>GPGSTEPFGLDRGLELDKVLHCYQMKELFLFVTWKGCSSIDAVPMKYIREAYPLQVIEFFQSGSGSGS[2x];>[2x]MENLAKIRMSQKLACWQQIL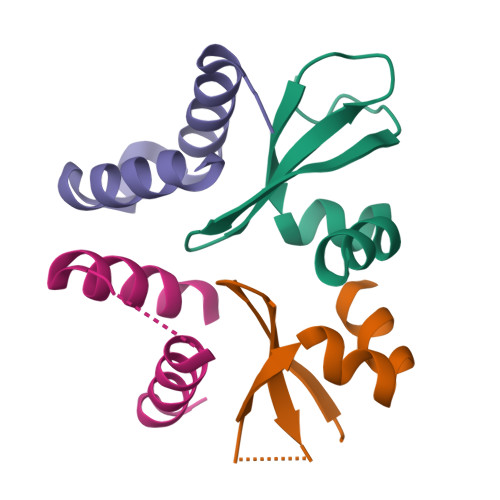TTLGTSSMSEQEWNTFFRGFLESWQNPYCIQTSCDPSIPL> PWEEPRSKSKICANVFCGAGRECAVTEKGEPTCLCIEQCKPHKRPVCGSNGKTYLNHCELHRDACLTGSKIQVD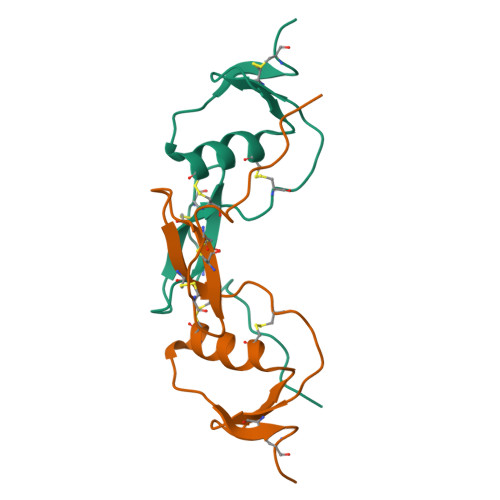YDGHCKE> ACDYTCGSNCY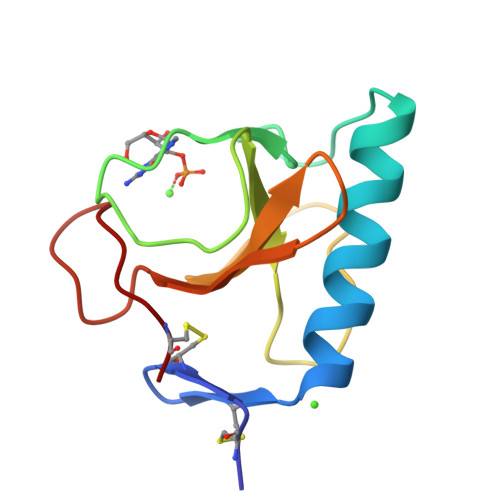SSSDVSTAQAAGYKLHEDGETVGSNSYPHKYNNYEGFDFSVSSPYYEWPILSSGDVYSGGSPGADRVVFNENNQLAGVITNTGASGNNFVECT(2~{S},3~{R},4~{S},5~{S},6~{S})-6-[(2-azanylhydrazinyl)methyl]oxane-2,3,4,5-tetrol 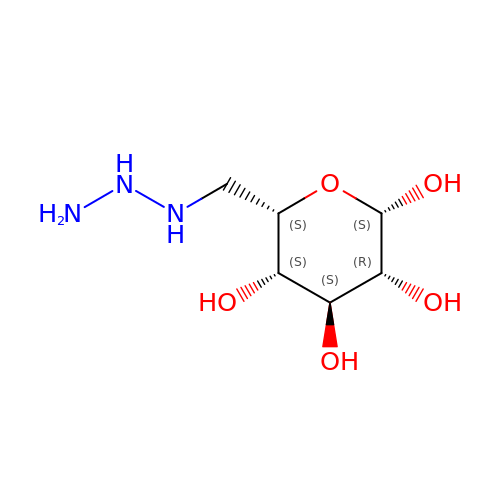| C6 H15 N3 O5 | HEZRRHKWEZVWNK-ZSNZIGRDSA-N> MAALDAALYEIYDGLILYQQRLKSLEGISPELGPALDALRYDMADFAILMAQAMEEGLDSLPQ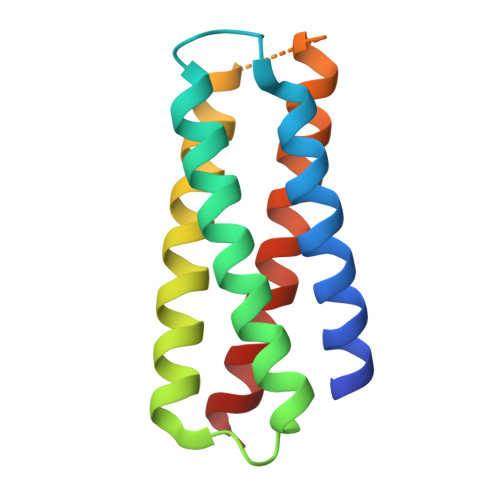SFLRKALEMIRKIQADAAALREKLAATYKGNDRAAAAQSIARKLEEMLEKAYQILRHLAAA>[2x]MAPVPEPEVVATPPADAGRGLIRVDSREIRHYSGTRKEPDYLVSRDNGKTWEMKAAPAGYPPNYGGIPKESPAIVRNPLTREFIRVQPIGGFVFLSRGGLDGKWLAVTNDGKLEEDWKDPEKRKNLKKLGGIMRTPVFVNKGRRVIVPFHNMGGGTKFHISDDGGLTWHVSRNGVTSPRHEARPPHQGVRWFNNAVEATVLEMKDGTLWALARTSQDQAWQAFSKDYGETWSKPEPSRFFGTLTMNTLGRLDDGTIVSLWTNTMALPENATAGNGTWEDVFTNRDSHHIAMSGDEGKTWYGFREIILDEHRNHPGYATLDGPEDRGKHQSEMVQLDKNRILISLGQHKNHRRLVIVDRRWVGAKTRATQTGKDLDSQWTIH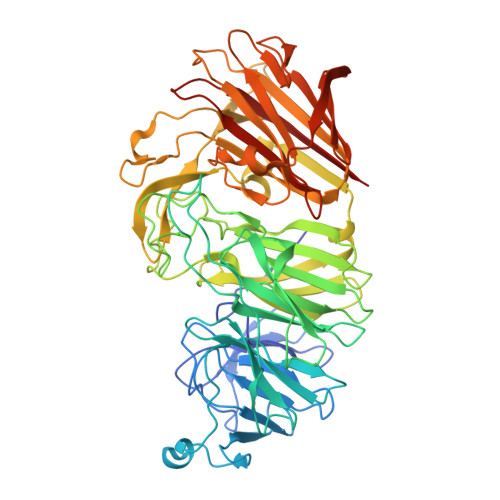TYIPQKKGHCSYNRKPSAELVQDPSGGTKKVLQIKRLDDPELVNEKSNVDYRNGGATWNFPNGTTGLVKFRFRVVDGEQADDSGLQVSLTDRLFNACDSTTKDYALFTFPIRLKPAPHLLLGMKKVPFTPGAWHEISLLWQGGQAVVSLDGKKAGTLKMANKSPNGASYIHFISTGSQPDAGILLDTVNARVKLEHHHHHH> ASWSHPQF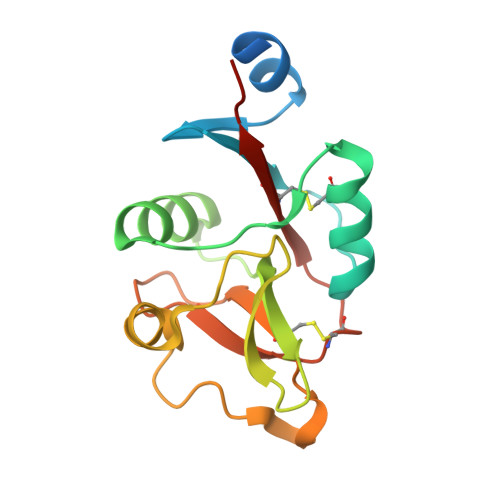EKIEGRMQNDILQVVSQGWKYFKGNFYYFSLIPKTWYSAEQFCVSRNSHLTSVTSESEQEFLYKTAGGLIYWIGLTKAGMEGDWSWVDDTPFNKVQSARFWIPGEPNNAGNNEHCGNIKAPSLQAWNDAPCDKTFLFICKRPYVPSEP>[2x]GMSIENLSSNKSFGGWHKQYSHV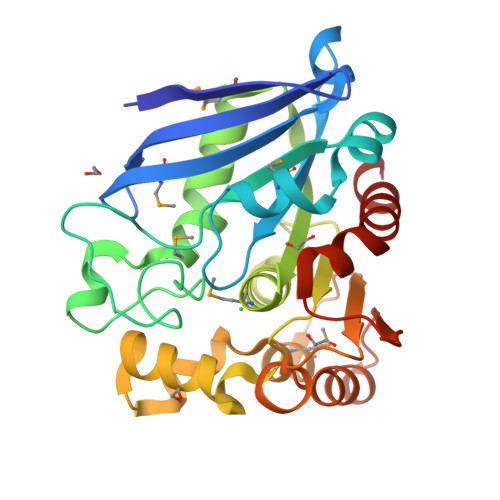SNTLNCAMRFAIYLPPQASTGAKVPVLYWLSGLTCSDENFMQKAGAQRLAAELGIAIVAPDTSPRGEGVADDEGYDLGQGAGFYVNATQAPWNRHYQMYDYVVNELPELIESMFPVSDKRAIAGHSMGGHGALTIALRNPERYQSVSAFSPINNPVNCPWGQKAFTAYLGKDTDTWREYDASLLMRAAKQYVPALVDQGEADNFLAEQLKPEVLEAAASSNNYPLELRSHEGYDHSYYFIASFIEDHLRFHSNYLNA> GSHMASMNYEIEVKDVEPIRVAFMHYKGPAAGASKVMPNVFKSIQGKANGAPFICYYVMDQQTMTGEMDLCVPTAENPVGNGIAVKDMPRIKAISA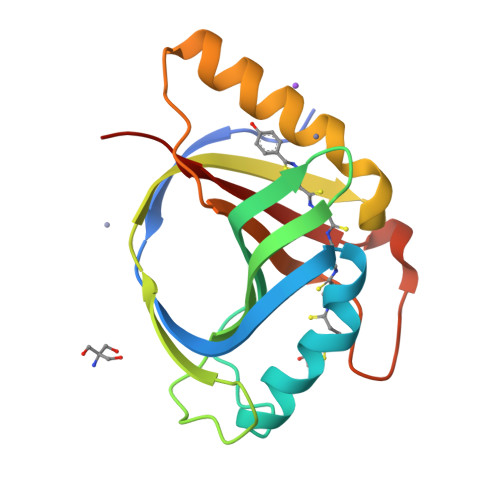THIGPYETMQPVYEAIESYAREKNLILQPPFREVFIKGPGMILKGNPNKYITEVLFPIKEE Microtubule (MT) nucleation is regulated by the γ-tubulin ring complex (γTuRC), conserved from yeast to humans. In budding yeast, homologues of the grip-containing proteins (GCPs) GCP2 and GCP3 (Spc97p and Spc98p) and two copies of γ–tubulin (Tub4p) form a 300 kDa complex (γTuSC). Spc110p, a distant pericentrin homologue, recruits this complex to the nuclear face of the spindle pole body (SPB), while Spc72p recruits it to the cytoplasmic face. In yeast, the CM1 motif is required for seven identical γTuSCs to helically assemble into a γTuRC at the SPB.

To validate this hypothesis, γ-tubulin was engineered with disulfides to stabilize a closed MT-like conformation (γTuRCSS), resulting in significantly enhanced MT nucleation. Realizing that this would require much higher resolution of Spc110p-γTuSC interactions, we focused on obtaining higher resolution structures of the ‘open’ (γTuRCWT) and disulfide trapped ‘closed’ (γTuRCSS) filaments containing Spc110p by collecting new datasets on a direct electron detector and incorporating symmetry expansion and 3D classification into the data processing pipeline. To improve the resolution, we performed symmetry expansion followed by focused classification of segments containing three adjacent γTuSCs. The resulting reconstructions were at a resolution of 3.6 Å and 3.0 Å for the γTuRCWT and γTuRCSS filaments, respectively (Figure 3—figure supplements 1–3). Indeed, the difference map revealed clear density extending from the NCC to a helical density that spans the inter-γTuSC interface and beyond. Based on the side-chain features, we were able to unambiguously assign CM1117-141 to the helical inter-γTuSC density. While the density connecting the Spc110pCM1 helix with Spc110pNCC was at a lower resolution, we were able to model residues Spc110p112-206 spanning the Spc110pCM1 and Spc110pNCC. Interestingly, a pair of helix-dipole/hydrogen bond interactions augment binding of the CM1 helix with Spc98p, with Spc98pD542 hydrogen bonding with the N-terminus of the Spc110pCM1 helix, and Spc110pK120 hydrogen bonding with the C-terminus of helix Spc98pH19. During the transition from the assembled open γTuRCWT to the engineered γTuRCSS closed conformation, the γ-tubulins on Spc97p and Spc98p slide past each other in roughly opposite directions, undergoing translations of ~6.9 Å and ~7.7 Å, respectively. Strikingly, our γTuRCSS structure reveals a cluster of phosphorylation sites, with many exhibiting in vivo phenotypes, that maps near the Spc110p:γTuSC interface in the Spc110pNCC region and near the loop connecting Spc110pNCC and Spc110pCM1.

>[4x]MGGEIITLQAGQCGNHVGKFLWSQLAKEHAIGTDGLSQLPDSSTERDDDTKPFFRENCRNKFTPRAIMMDSEPSVIADVENTFRGFFDPRNTWVASDGASAGNSWANGYDIGTRNQDDILNKIDKEIDSTDNFEGFQLLHSVAGGTGSGLGSNLLEALCDRYPKKILTTYSVFPARSSEVVVQSYNTILALRRLIEDSDATVVFDNASLLNISGKVFRNPNIDLQHTNQLISTIISSVTNSIRFPSYMYSSMSSIYSTLIPSPELHFLSPSFTPFTSDYIHDDIAHKCHSSYDVMLDLLDPSNSLVSTAMNNPTYFNVYNTIIGNVEPRQISRAMTKLQQRIKFPSWSSSAMHVNIGRRSPYLPLQPNENEVSGMMLSNMSTVVNVFENACNTFDKVFAKGAFLNNYNVGDLFQSMQNVQDEFAESREVVQSLMEDYVAAEQDSYLDDVLVDDENMVGELEEDLDADGDHKLV;>[2x]MEIKEVDDRAELLRYTNNIPLLGKLVNHQPLWSTNPKLKSFSLEKISAPDQRRVQEALVVKDLLNVLIGLEGTYIRYFNDYEPSDPETPIEFKIAKKMDPSFKTFSRRIVRYGKQYMILTRAYEKWSDTSFGMVLQRFAYEIRRFLEDVYLKTLVERLERDFNKVPNFSIRELEQIINETEVNKQMELLYNIYEEIFREIEERRTNQSSQEDFNNFMDSMKNESSLHLRLMVAFDTTVYPVPKGGAILKIFQQKILENLGDRSSVMFLKKLLNNISQDYCTMLYEWLTQGILNDPYQEFMTYDDLEGKTDNIFDTRDRAWDTQYFIRKDVLLRDCDSEEDKNLLFKMLRTGILLKVVRASLQIPTIPSNSSDITIQEINDFADLMEGSNLELYVDKCYSRANEIFLKLFFQGYDLINVLKHLQQIFLGYQSGHNVLKFLTKNMGELTKHYRNDNNANYDKLLQNFELERQSENPNNLMRQLLMIQFDTETLPQVLSHYLQIYPEVPENNSANDDSDPLMHANNFKNMNAILFDELSKERTGAYHGSNLELYTPKSAIYHLKFDINIPYPLNIIISRTCMIKYQIILRYQLVLQYHSRLLDETWMDLNKTPSWKYRGYSHTVKRRIVRATRVLHAKMNHFIKTIMEYFNQNVIDKEVYSLEKCYRNPTLAVAIQNELEGGLTNIMTNRCLSDLIPLQLQIFDIVYKFCKFIKSMRAKLCQLDPVLYEKHKSGMMKTLNEGYRTNNGGQEDVGYQEDAALELIQKLIEYISNASSIFRKCLINFTQELSTEKFDFYDSSSVDAAGIERVLYSIVPPRSASASSQR;>MELEPTLFGIIEALAPQLLSQSHLQTFVSDVVNLLRSSTKSATQLGPLIDFYKLQSLDSPETTIMWHKIEKFLDALFGIQNTDDMVKYLSVFQSLLPSNYRAKIVQKSSGLNMENLANHEHLLSPVRAPSIYTEASFENMDRFSERRSMVSSPNRYVPSSTYSSVTLRQLSNPYYVNTIPEEDILKYVSYTLLATTSALFPFDHEQIQIPSKIPNFESGLLHLIFEAGLLYQSLGYKVEKFRMLNISPMKKALIIEISEELQNYTAFVNNLVSSGTVVSLKSLYREIYENIIRLRIYCRFTEHLEELSGDTFLIELNIFKSHGDLTIRKIATNLFNSMISLYYEYLMNWLTKGLLRATYGEFFIAENTDTNGTDDDFIYHIPIEFNQERVPAFIPKELAYKIFMIGKSYIFLEKYCKEVQWTNEFSKKYHVLYQSNSYRGISTNFFEIINDQYSEIVNHTNQILNQKFHYRDVVFALKNILLMGKSDFMDALIEKANDILATPSDSLPNYKLTRVLQEAVQLSSLRHLMNSPRNSSVINGLDARVLDLGHGSVGWDVFTLDYILYPPLSLVLNVNRPFGRKEYLRIFNFLWRFKKNNYFYQKEMLKSNDIIRSFKKIRGYNPLIRDIINKLSRISILRTQFQQFNSKMESYYLNCIIEENFKEMTRKLQRTENKSQNQFDLIRLNNGTIELNGILTPKAEVLTKSSSSKPQKHAIEKTLNIDELESVHNTFLTNILSHKLFATNTSEISVGDYSGQPYPTSLVLLLNSVYEFVKVYCNLNDIGYEIFIKMNLNDHEASNGLLGKFNTNLKEIVSQYKNFKDRLYIFRADLKNDGDEELFLLSKSLR[2x];>[4x]MDEASHLPNGSLKNMEFTPVGFIKSKRNTTQTQVVSPTKVPNANNGDENEGPVKKRQRRSIDDTIDSTRLFSEASQFDDSFPEIKANIPPSPRSGNVDKSRKRNLIDDLKKDVPMSQPLKEQEVREHQMKKERFDRALESKLLGKRHITYANSDISNKELYINEIKSLKHEIKELRKEKNDTLNNYDTLEEETDDLKNRLQALEKELDAKNKIVNSRKVD>[2x]GSHMSDSNTITSFQVDCYLWHIRKLLSMRDMCDAPFDDRLRRDQKALKGRGSTL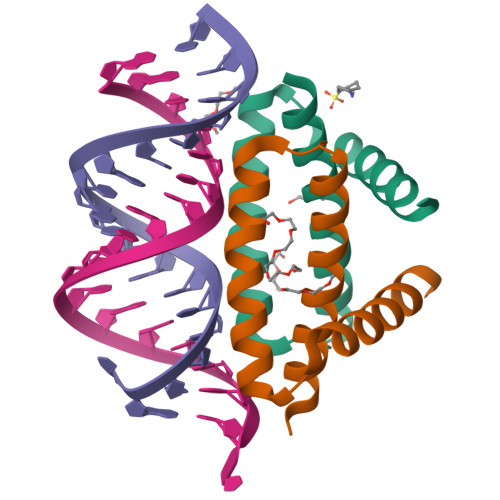GLDLRVATMEGKKIVEDILKSET> ELEGCETAILFPMRSKKIFGSVHPVRPMRLESFSACIWVKATDVLNKTILFSYGTKRNPYEIQLYLSYQSIVFVVGGEENKLVAEAMVSLGRWTHLCGTWNSEEGLTSLWVNG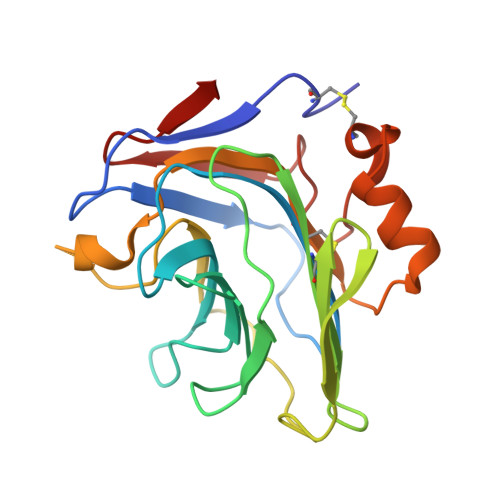ELAATTVEMATGHIVPEGGILQIGQEKNGCCVGGGFDETLAFSGRLTGFNIWDSVLSNEEIRETGGAESCHIRGNIVGWGVTEIQPHGGAQYVS> MAIVGVGIDLVSIPDFAEQVDRPGTVFAETFTPGERRDAADKSSSAARHLAARWAAKEAVIKAWSSSRFSKRPALPEGIHRDIEVVTDMWGR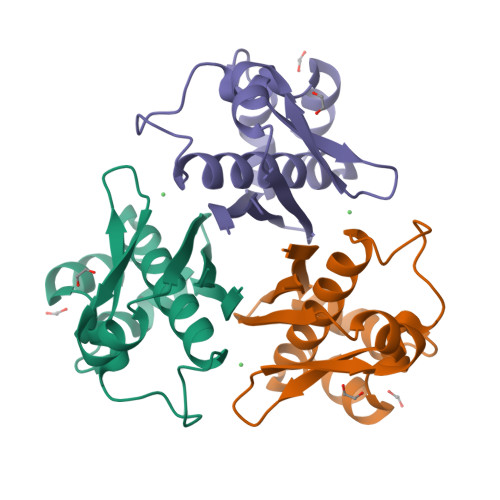PKVRLSGEIAKHLEDVTIHVSLTHEDQTAAAVAIIEEP> MDENLEQVSGIIGNLRHMALDMGNEIDTQNRQIDRIMEKADSNKTRIDEANQR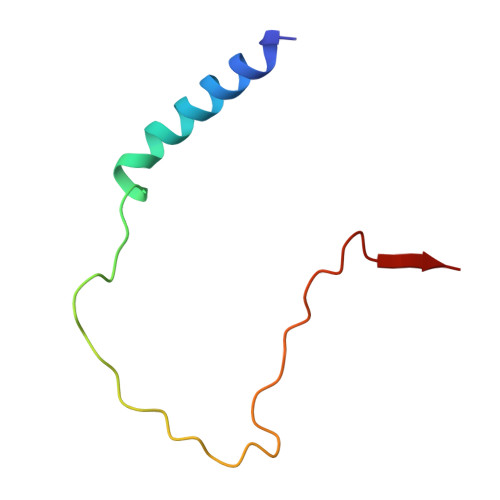ATKMLG>SNAMKRKILITGGTGMLGAYVTSALKDTDYNVIVTERNTLNLSVPEAIFSYITAEKPDVILHFAAETDVDLCEREPARAGIYNHLATEQIAQAAKFCGAWLLYLSSSNVFGGEGKLSYNELDIPLPMNYYGRSKLIGESSVRNACTNNHLIIRAGWMIGGGPDKDHKFVGKIIQQIKAGSTSIKAVSDRLGSITSAMQLCNFIIWAINKRHTGTLHFASSGTISRFDIACAIGDLLNFKGDIIPVHSSVFPLSAPRPYSEGIESIYMSILSDAPKPSLWKSD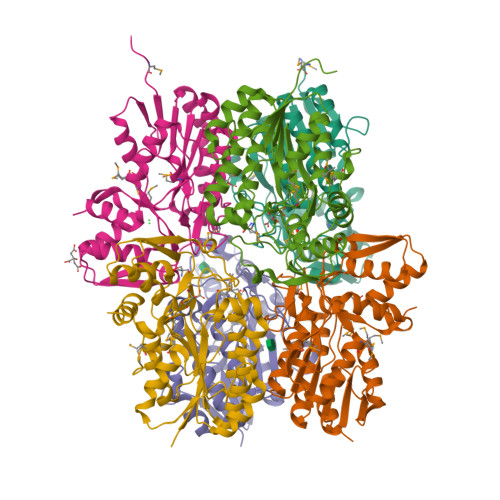LAKYVGTFLV[6x]>ARSEKRVPMTRLRKRVAERLLEAKNSTAMLTTFNEVNMKPIMDLRKQYGEAFEKRHGIRLGFMSFYVKAVVEALKRYPEVNASIDGDDVVYHNYFDVSMAVSTPRGLVTPVLRDVDTLGMADIEKKIKELAVKGRDGKLTVEDLTGGNFTITNGGVFGSLMSTPIINPPQSAILGMHAIKDR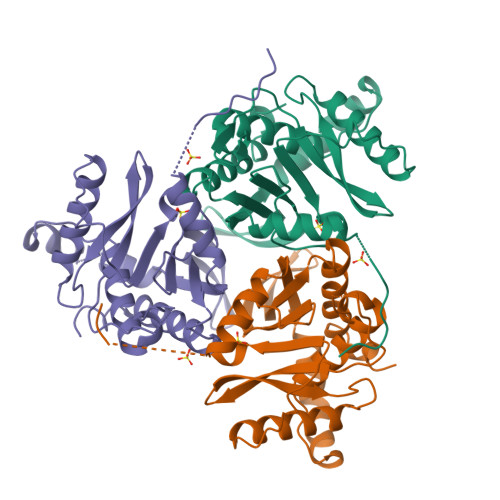PMAVNGQVEILPMMYLALSYDHRLIDGRESVGFLVTIKELLEDPTRLLLDV[3x]4-(1-methyl-3,6-dihydro-2H-pyridin-4-yl)phenol | C12 H15 N O | 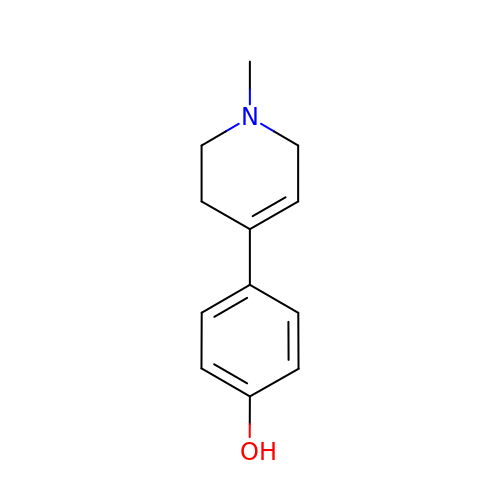GIGCUVKCMPXMAZ-UHFFFAOYSA-N>XPPGPPGEPGMRGLPGAVGP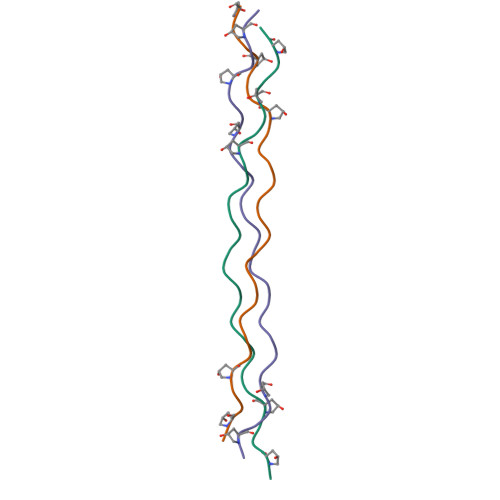PGPPGPPG[6x]BIS-NORESEROLINE 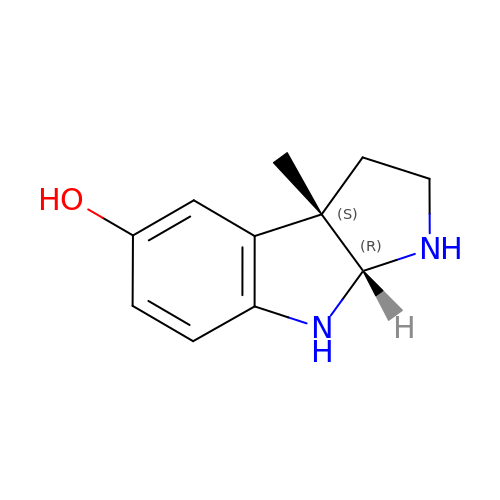| C11 H14 N2 O | BLEHTFVVORLVPX-MNOVXSKESA-N(4S)-6-[([1,1'-biphenyl]-2-yl)oxy]-3-chloro[1,2,4]triazolo[4,3-b]pyridazine | C17 H11 Cl N4 O | 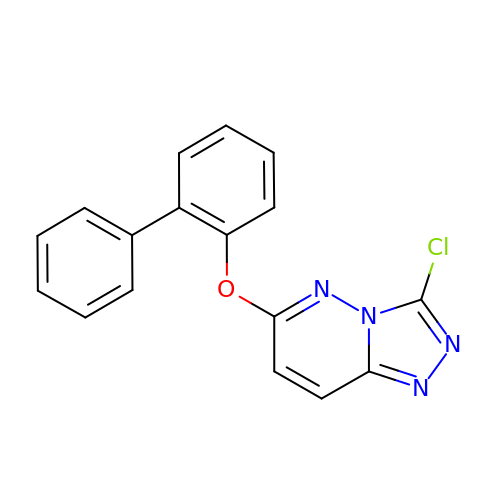XWHTYUYQMHCFMT-UHFFFAOYSA-N> AWPKVQPEVNIGVVGHVDHGKTTLVQAITGIWTSKKLGYAETNIGVCESCKKPEAYVTEPSCKSCGSDDEPKFLRRISFIDAPGHEVLMATMLSGAALMDGAILVVAANEPFPQPQTREHFVALGIIGVKNLIIVQNKVDVVSKEEALSQYRQIKQFTKGTWAENVPIIPVSALHKINIDSLIEGIEEYIKTPYRDLSQKPVMLVIRSFDVNKPGTQFNELKGGVIGGSIIQGLFKVDQEIKVLPGLRVEKQGKVSYEPIFTKISSIRFGDEEFKEAKPGGLVAIGTYLDPSLTKADNLLGSIITLADAEVPVLWNIRIKYNLLERVVGAKEMLKVDPIRAKETLMLSVGSSTTLGIVTSVKKDEIEVELRRPVAVWSNNIRTVISRQIAGRWRMIGW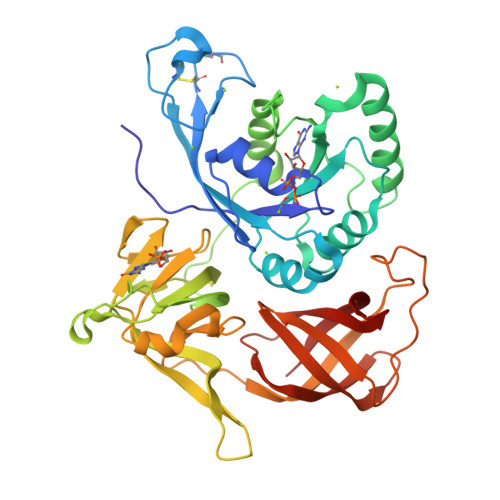GLVEI>MHGSNKLPGFATRAIHHGYDPQDHGGALVPPVYQTATFTFPTVEYGAACFAGEQAGHFYSRISNPTLNLLEARMASLEGGEAGLALASGMGAITSTLWTLLRPGDEVLLGNTLYGHTFAFLHHGIGEFGVKLRHVDMADLQALEAAMTPATRVIYFESPANPNMHMADIAGVAKIARKHGATVVVDNTYCTPYLQRPLELGADLVVHSATKYLSGHGDITAGIVVGSQALVDRIRLQGLKDMTGAVLSPHDAALLMRGIKTLNLRMDRHCANAQVLAEFLARQPQVELIHYPGLASFPQYTLARQQMSQPGGMIAFELKGGIGAGRRFMNALQLFSRAVSLGDAESLAQHPASMTHSSYTPEERAHYGISEGLVRLSVGLEDIDDLLADVQQA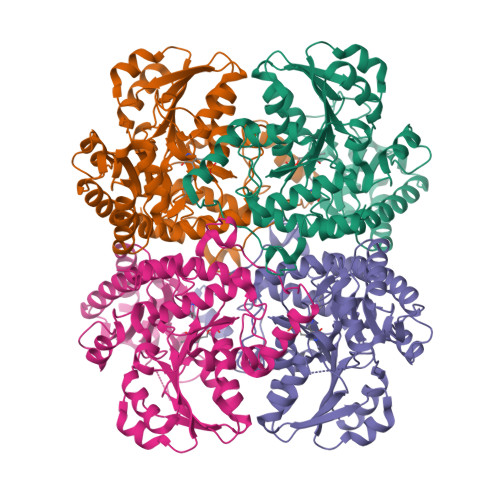LKASA[4x]>[2x]LSTCTTLDFGHIKKKRVEAIRGQILSKLRLTSPPEPTVMTHVPYQVLALYNSTRELLEEMHGEREEGCTQENTESEYYAKEIHKFDMIQGLAEHNELAVCPKGITSKVFRFNVSSVEKNRTNLFRAEFRVLRVPNPSSKRNEQRIELFQILRPDEHIAKQRYIGGKNLPTRGTAEWLSFDVTDTVREWLLRRESNLGLEISIHCPCHTFQPNGDILENIHEVMEIKFKGVDNEDDHGRGDLGRLKKQKDHHNPHLILMMIPPHRLDNPGQGGQRKKRALDTNYCFRNLEENCCVRPLYIDFRQDLGWKWVHEPKGYYANFCSGPCPYLRSADTTHSTVLGLYNTLNPEASASPCCVPQDLEPLTILYYVGRTPKVEQLSNMVVKSCKCS;> HQDKVPCKMVD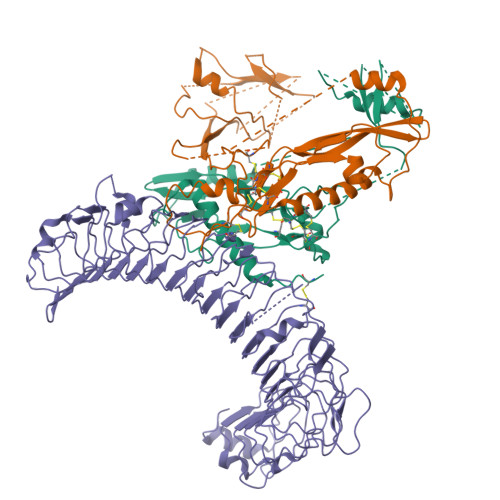KKVSCQVLGLLQVPSVLPPDTETLDLSGNQLRSILASPLGFYTALRHLDLSTNEISFLQPGAFQALTHLEHLSLAHNRLAMATALSAGGLGPLPRVTSLDLSGNSLYSGLLERLLGEAPSLHTLSLAENSLTRLTRHTFRDMPALEQLDLHSNVLMDIEDGAFEGLPRLTHLNLSRNSLTCISDFSLQQLRVLDLSCNSIEAFQTASQPQAEFQLTWLDLRENKLLHFPDLAALPRLIYLNLSNNLIRLPTGPPQDSKGIHAPSEGWSALPLSAPSGNASGRPLSQLLNLDLSYNEIELIPDSFLEHLTSLCFLNLSRNCLRTFEARRLGSLPCLMLLDLSHNALETLELGARALGSLRTLLLQGNALRDLPPYTFANLASLQRLNLQGNRVSPCGGPDEPGPSGCVAFSGITSLRSLSLVDNEIELLRAGAFLHTPLTELDLSSNPGLEVATGALGGLEASLEVLALQGNGLMVLQVDLPCFICLKRLNLAENRLSHLPAWTQAVSLEVLDLRNNSFSLLPGSAMGGLETSLRRLYLQGNPLSCCGNGWLAAQLHQGRVDVDATQDLICRFSSQEEVSLSHVRPEDCEKGGLKNIN>[4x]GSHNMAEMVETVCGPVPVEQLGKTLIHEHFLFGYPGFQGDVTRGTFREDESLRVAVEAAEKMKRHGIQTVVDPTPNDCGRNPAFLRRVAEETGLNIICATGYPYEGEGAPPYFQFRRLLGTAEDDIYDMFMAELTEGIADTGIKAGVIKLASSKGRITEYEKMFF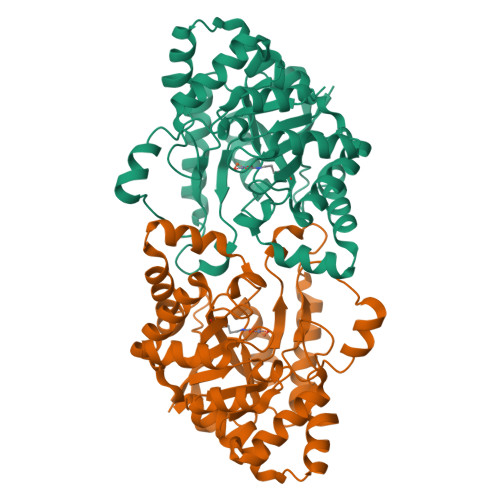RAAARAQKETGAVIITHTQEGTMGPEQAAYLLEHGADPKKIVIGHMCGNTDPDYHRKTLAYGVYIAFDRFGIQGMVGAPTDEERVRTLLALLRDGYEKQIMLSHDTVNVWLGRPFTLPEPFAEMMKNWHVEHLFVNIIPALKNEGIRDEVLEQMFIGNPAALFSA The Rab11 subfamily plays important roles in specific trafficking events such as exocytosis, endosomal recycling, and cytokinesis. SH3BP5 and SH3BP5-like (SH3BP5L) proteins have recently been found to serve as guanine nucleotide exchange factors (GEF) for Rab11. SH3BP5 exhibits a V-shaped structure comprising two coiled coils. The coiled coil composed of α1, and α4 is solely responsible for the Rab11a binding and GEF activity.

Because computational secondary structure prediction assigned the N- and C-terminal regions as mostly disordered regions, we selected the central helical region for crystallography. We found that the R260A/R261A/R262A triple mutation reduced the degradation and obtained diffraction-quality crystals. This construct of SH3BP5 (41–266; R260A/R261A/R262A) is hereafter referred to as SH3BP5-RA. In addition, the M167A mutation was introduced to improve the solubility of the selenomethionine (SeMet)-labeled SH3BP5-RA (SeMet SH3BP5-RA/M167A), which was used for phase determination by the single-wavelength anomalous diffraction method. Finally, we determined the crystal structures of SeMet SH3BP5-RA/M167A in two different crystal forms (I41 and P41) and native SH3BP5-RA at 3.35, 3.6, and 3.8 Å resolutions, respectively. The asymmetric units of the I41 and P41 crystals contain one and two SH3BP5 molecules, respectively. Therefore, we obtained five different apo-SH3BP5 structures in total (i.e., one from I41 SeMet SH3BP5-RA/M167A, two from P41 SeMet SH3BP5-RA/M167A, and two from P41 native SH3BP5-RA). Although these five apo-SH3BP5 structures exhibit a similar V-shaped conformation, the superposition of these five apo-SH3BP5 structures using α1 as the reference shows some flexibility of the conformation. The hinge region of the V shape contains staggered hydrophobic interactions so as to maintain the V shape.

>SHVDPRIQGELEKLNQSTDDINRRETELEDARQKFRSVLVEATVKLDELVKKIGKAVEDSKPYWEARRVARQAQLEAQKATQDFQRATEVLRAAKETISLAEQRLLEDDKRQFDSAWQEMLNHATQRVAEAEQTKTRSELVHKETAARYNAAMGRMRQLEKKLKRAINKSKPYFELKAKYYVQLEQLKKTVDDLQAKLTLAKGEYKMALKNLEMISDEIHEAAASSAM[2x]> MAPSRLCVYCADVCPDRLRCAAWLLATGIFLLLAGCSEAKAPTALERVQKEGVLRVITRNSPATYFQDRNGETGFEYELAKRFAERLGVELKIETADNLDDLYAQLSREGG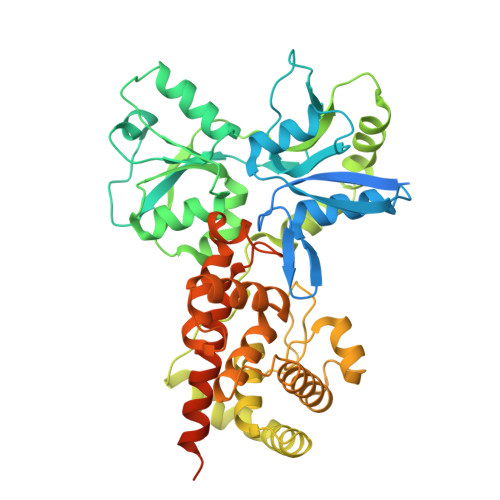PALAAAGLTPGRDDDASVRYSHTYLDVTPQIIYRNGQQRPTRPEDLVGKRIMVLKGSSHAEQLAELKKQYPELKYEESDAVEVVDLLRMVDVGDIDLTLVDSNELAMNQVYFPNVRVAFDFGEARGLAWALPGGDDDSLMNEVNAFLDQAKKEGLLQRLKDRYYGHVDVLGYVGAYTFTQHLQQRLPRYESHFKQSGKQKDTDWRLLAAIGYQESLWQPGATSKTGVRGLMMLTNRTAQAMGVSNRLDPKQSIQGGSKYFVQIRSELPESIKEPDRSWFALAAYNIGGAHLEDARKMAEKEGLNPNKWLDVKKMLPRLAQKQWYAKTRYGYARGGETVHFVQNVRRYYDILTWVTQPQMEGSQIAESGLHLPGVNKTRPEEDSGDEKL>MSLQFIGLQRRDVVALVNFLRHLTQKPDVDLEAHPKILKKCGEKRLHRRTVLFNELMLWLGYYRELRFHNPDLSSVLEEFEVRCVAVARRGYTYPFGDRGKARDHLAVLDRTEFDTDVRHDAEIVERALVSAVILAKMSVRETLVTAIGQTEPIAFVHLKDTEVQRIEENLEGVRRNMFCVKPLDLNLDRHANTALVNAVNKLVY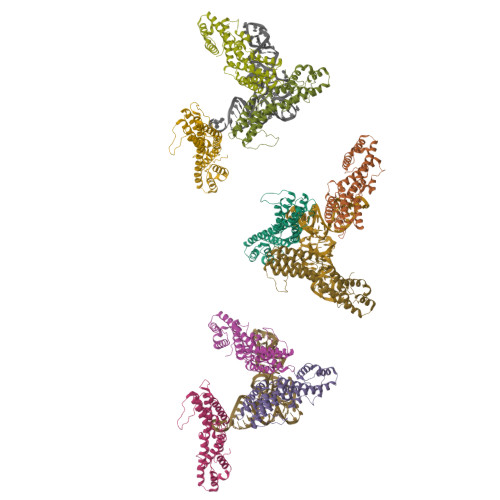TGRLIMNVRRSWEELERKCLARIQERCKLLVKELRMCLSFDSNYCRNILKHAVENGDSADTLLELLIEDFDIYVDSFPQS[9x]>[2x]XHLTIHTWPEYGYAAIDLFTCGEDVDPWKAFEHLKKALKAKRVHVVEHERGRYDEIGIPEDSPHKAAV;>[2x]MKSLGRHLVAEFYECDRE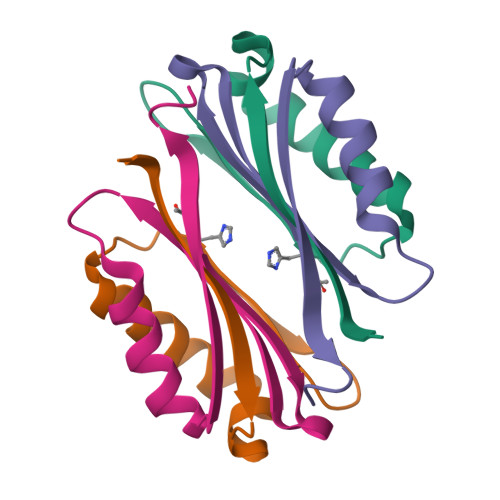VLDNVQLIEQEMKQAAYESGATIVTSTFHRFLPYGVSGVVVISE>[2x]AGAGAMNASPQLDHHTELHAAPPLWRPGRVLARLREHQPGPVHIIDPFKVPVTEAVEKAAELTRLGFAAVLLA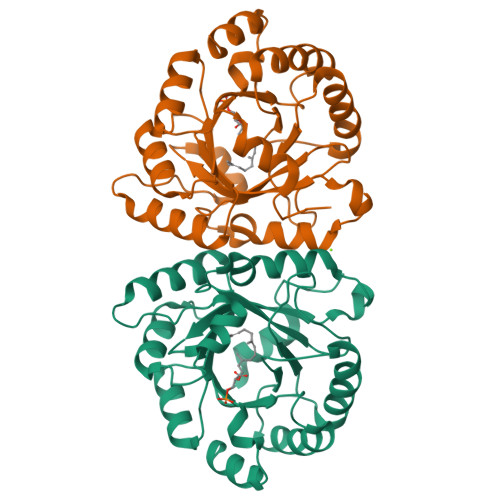STDYESFESHMEPYVAAVKAATPLPVVLHFPPRPGAGFPVVRGADALLLPALLGSGDDYFVWKSFLETLAAFPGRIPREEWPELLLTVALTFGEDPRTGDLLGTVPVSTASTEEIDRYLHVARAFGFHMVYLYSRNEHVPPEVVRHFRKGLGPDQVLFVSGNVRSGRQVTEYLDSGADYVGFAGALEQPDWRSALAEIAGRRPAAPARPGSGR>GSMQPDMSLNVIKMKSSDFLESAELDSGGFGKVSLAFHRTQGLMIMKTVYKGPNCIEHNEALLEEAKMMNRLRHSRVVKLLGVIIEEGKYSLVMEYMEKGNLMHVLKAEMSTPLSVKGRIILEIIEGMAYLHGKGVIHKDLKPENILVDNDFHIKIADLGLASFKMWSKLNNEEHNELREVDGTAKKNGGTLYYMAPEHLNDVNAKPTEK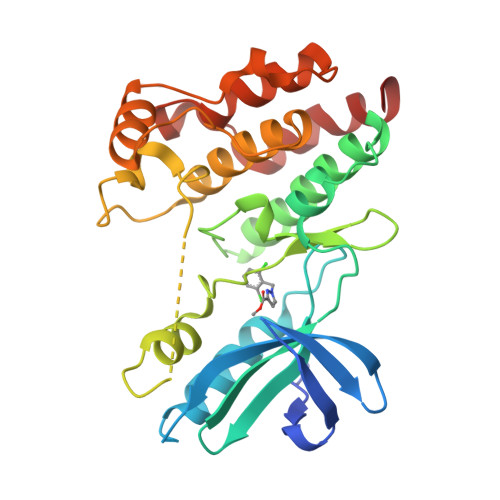SDVYSFAVVLWAIFANKEPYENAIAEQQLIMAIKSGNRPDVDDITEYCPREIISLMKLCWEANPEARPTFPGIEEKFRPFYLSQLE[4x]> MQKLSRVVCNRLVRFHGTVAASAGGKRYDLFGYEVSVATGPFIEEIKKAQFYDD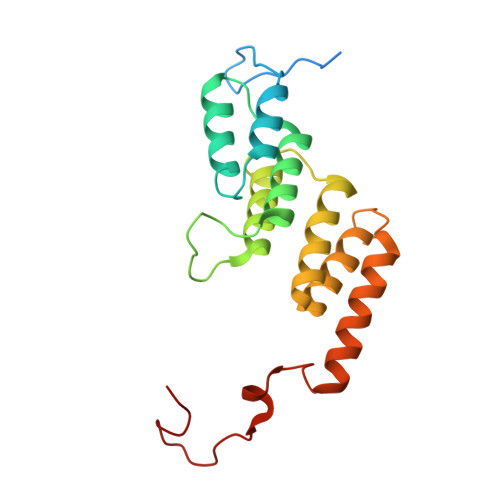AGEVIVKMNLANTPPDLQTYNAVLERILNCKSKRSQPVKGENKFAAMMDILEEMDARSGIKPNAESWGYVLKELVQAGDFRLGWVCIAGMKSLGITPDQALVDANEANAAKAKAAGTDFPAYLKKAAPESFDTKAWGI>[2x]ACYCRIPACI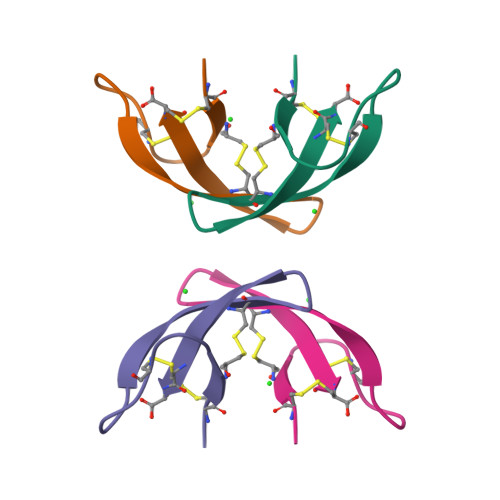AGERRYGTCIYQGRLWAFCC> SEESRESPAEHGYYMPAEWDSHAQTWIGWPERQDNWRHNALPAQRVFAGVAKAISKF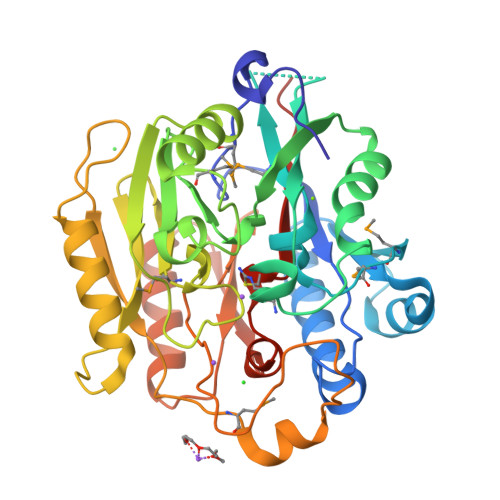EPVTVCASPAQWENARKQLPEDIRVVEMSMNDSWFRDSGPTFIVRKRPVKLSSLNRNIAGIDWNFNAWGGANDGCYNDWSHDLLVSRKILALERIPRFQHSMILEGGSIHVDGEGTCLVTEECLLNKNRNPHMSKEQIEEELKKYLGVQSFIWLPRGLYGDEDTNGHIDNMCCFARPGVVLLSWTDDETDPQYERSVEALSVLSNSIDARGRKIQVIKLYIPEPLYMTEEESSGITQDGEAIPRLAGTRLAASYVNFYIANGGIIAPQFGDPIRDKEAIRVLSDTFPHHSVVGIENAREIVLAGGNIHCITQQQPAEPTSVAENGH>[4x]MAEAAAAAAAAAAAGETSASSGSAAERDPDQDRAGRRLRVLSGHLLGRPQEALSTNECKARRAASAATAAPTATPAAPESGIIPKKRQELMKWNGWGYNDSKFFLNKKGQLELTGKRYPLSGVALPTFKDWIQNTFGINLDHKTTSKASLNPSDTPPSIVNEDFLHELKKTNISYSQEADDRVFRAHGHCLHEIFLLREGMFERIPDIVLWPTCHDDVVKIVNLACKYNLCIIPIGGGTSVSYGLMCPADETRTIISLDTSQMNRILWVDENNLTAHVEAGITGQELERQLKESGYCTGHEPDSLEFSTVGGWISTRASGMKKNIYGNIEDLVVHMKVVTPRGVIEKSCQGPRMSTGPDIHHFIMGSEGTLGVITEATIKIRPTPEYQKYGSVAFPNFEQGVACLREIAKQRCAPASIRLMDNQQFQFGHALKPQVSSIFTSFLDGLKKFYITKFKGFDPNQLSVATLLFEGDREKVLQHEK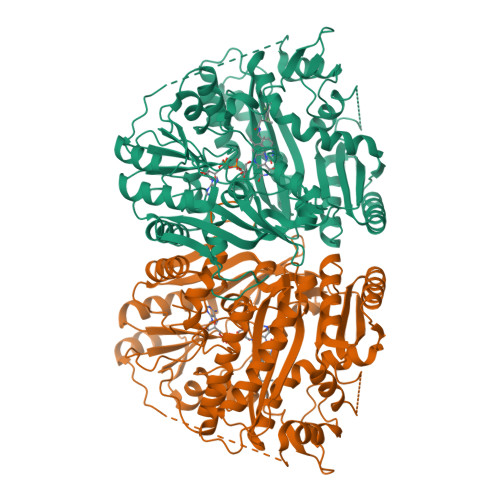QVYDIAAKFGGLAAGEDNGQRGYLLTYVIAYMRDLGLEYYIIGESFETSAPWDRVVDLCRNVKERIRRECKEKGVQFPPLSTCRVTQTYDAGACIYFYFAFNYRGISDPLAVFEQTEAAAREEILANGGSLSHHHGVGKLRKQWLKESISDVGFGMLKSVKDYVDPTNIFGNRNLL2-{2-[(3,5-dimethylphenyl)amino]pyrimidin-4-yl}-N-[(1S)-2-hydroxy-1-methylethyl]-4-methyl-1,3-thiazole-5-carboxamide 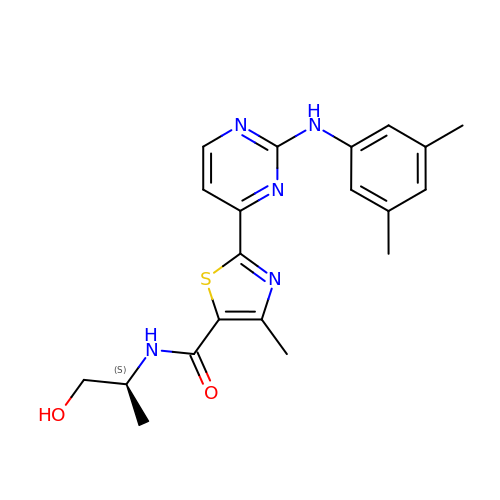| C20 H23 N5 O2 S | PEGXADGTBNRSGV-ZDUSSCGKSA-N>GSMASSSTAYYLKDAGFHIRNIPKAWNDWNLFHVFQNFGKVSYCRVVGQSNDGQVQLGFVNMMSVADADEVRKNMNDGNLIGENFTLKVTDHKN[2x];>[2x]MEGDIHMQENMLKISGYPGMLNTFGIAQLLTPYRVNGITMTGAQSAVVALENKFQVYQAVQDFNGKKLDRNHKLQVSSLVVSSPAVPLE

By using functional proteomics, we and another group independently identified a piRNA biogenesis and chromosome segregation (PICS) complex (also named as PETISCO) that plays important roles in 21U-RNA biogenesis, chromosome segregation and cell division. The PICS complex is composed of TOFU-6, PICS-1 (also names as PID-3), ERH-2 and two mutually exclusive factors, PID-1 and TOST-1. The PID-1 containing complex is functional in piRNA maturation and processes piRNA precursors at 5′ termini via its association with IFE-3, while the TOST-1 containing form is essential for chromosome segregation and cell division in embryos. Complemented by biochemical and mutagenesis experiments, our structural biology data support that PICS is an octamer composed of two copies of each subunit, and unveil the assembly interface within PICS complex.

Consistent with previous work, PICS-1(PID-3) and TOFU-6 interact with each other via RRM domains, which were previously identified as the RNA binding modules. Given that the two structures are almost identical, the native one was used for structural analysis. For one half of the interface, Phe217A is buried in a hydrophobic pocket composed of Phe217B, Ala220B, V228B, and I231B. Altogether, both hydrophobic and electrostatic interactions contribute to the dimerization and the other half of the dimerization interface could be obtained via the symmetry. TOFU-6C primarily interacts with PICS-1A through α1-β2 of TOFU-6C, and α2 and a C-terminal fragment of PICS-1A. α1 of TOFU-6C interacts with α2 of PICS-1A via both hydrophobic and electrostatic interactions. Specifically, Trp27, Phe30, His31, and Cys42 of TOFU-6C, make hydrophobic interactions with Lys246, Phe247, and Tyr250 of PICS-1A. Asp26 and Gln34 of TOFU-6C form salt bridges with Lys246 and Gln254 of PICS-1A, respectively. In addition, α1 of TOFU-6C also interacts with the PICS-1(PID-3) C-terminus via electrostatic interactions. TOFU-6C also contacts with the other protomer of PICS-1(PID-3) (PICS-1B). For cells with tofu-6 mutants, PICS-1(PID-3) failed to accumulate at the perinuclear granules in the germline, but a large fraction of the protein changed the localization from the cytoplasm to nucleoplasm in germline and embryos. Taken together, the localization of PICS-1(PID-3) in the cytosol depends on TOFU-6, and the TOFU-6/PICS-1 interaction is critical for both proteins to associate with perinuclear granules.>QAFRKFTKSERSKDLIKEAILDNDFMKNLELSQIQEIVDCMYPVEYGKDSCIIKEGDVGSLVYVMEDGKVEVTKEGVKLCTMGPGKVFGELAILYN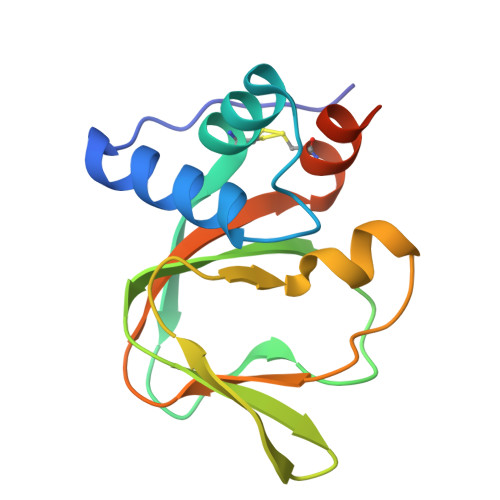CTQTATVKTLVNVKLWAIDRQCFQTIMMRTGLIKHTEY[2x]>MGSDKIHHHHHHMSNHSSSIPELSDNGIRYYQTYNESLSLWPVRCKSFYISTRFGQTHVIASGPEDAPPLVLLHGALFSSTMWYPNIADWSSKYRTYAVDIIGDKNKSIPENVSGTRTDYANWLLDVFDNLGIEKSHMIGLSLGGLHTMNFLLRMPERVKSAAILSPAETFLPFHHDFYKYALGLTASNGVETFLNWMMNDQNVLHPIFVKQFKAGVMWQDGSRNPNPNADGFPYVFTDEELRSARVPILLLLGEHEVIYDPHSALHRASSFVPDIEAEVIKNAGHVLSMEQPTYVNERVMRFFN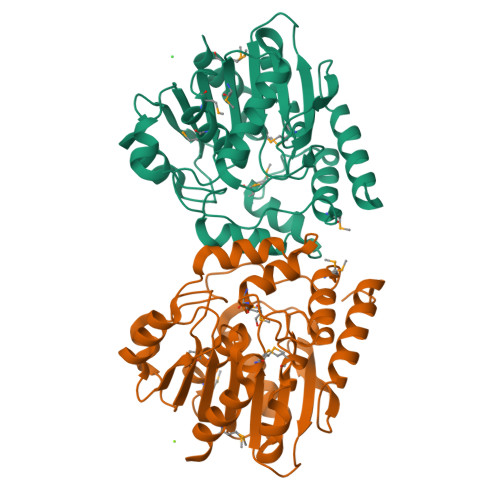A[4x]>MSNLLTVHQNLPALPVDATSDEVRKNLMDMFRDRQAFSEHTWKMLLSVCRSWAAWCKLNNRKWFPAEPEDVRDYLLYLQARGLAVKTIQQHLGQLNMLHRRSGLPRPSDSNAVSLVMRRIRKENVDAGERAKQALAFERTDFDQVRSLMENSDRCQDIRNLAFLGIAYNTLLKIAEIARIRVKDISRTDGGRMLIHIGRTKTLVSTAGVEKALSLGVTKLVERWISVSGVADDPNNYLFCRVRKNGVAAPSATSQLSTRALEGIFEATHRLIYGAKDDSGQRYLAWSGHSARVGAARDMARAGVSIPEIMQAGGWTNVNIVMN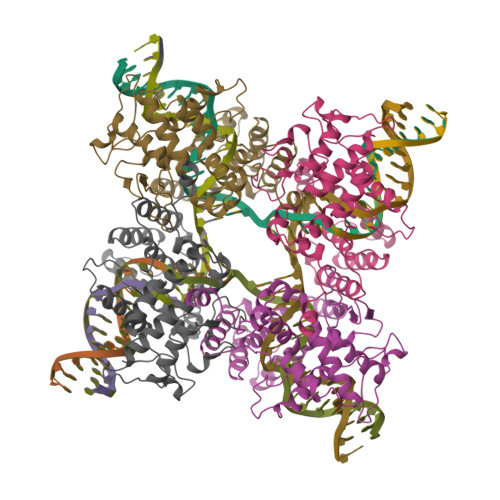YIRNLDSETGAMVRLLEDGD[2x]> STRRATSLELPMAMRFRHLKKTSKEAVGVYRSAIHGRGLFCKRNIDAGEMVIEYSGIVIRSVLTDKREKFYDGKGIGCYMFRMDDFDVVDAT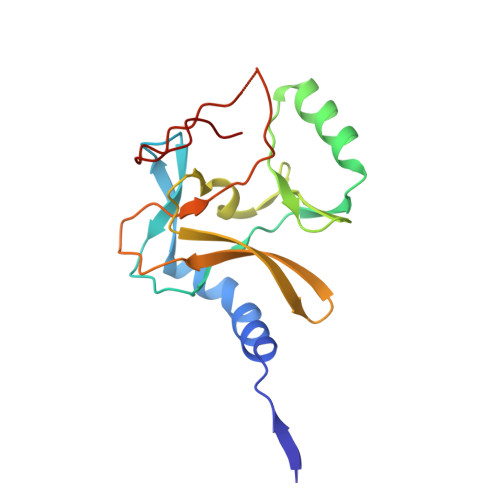MHGNAARFINHSCEPNCFSRVIHVEGQKHIVIFALRRILRGEELTYDYKFPIEDASNKLPCNCGAKRCRRFLN Extensive studies have identified that many RNA-binding proteins, such as FUS, hnRNPA1, and TDP43, largely contribute to this conditional cellular compartmentation. These proteins commonly contain low complexity (LC) domains that can drive the full-length proteins to undergo liquid–liquid phase separation (LLPS) via weak multivalent interactions. In this work, we directly visualize temperature-sensitive amyloid fibrils in the liquid-like droplets of hnRNPA1 by transmission electron microscopy (TEM). Our work bridges the liquid phase and solid phase of hnRNPA1 and illuminates the functional role of reversible amyloids in the assembly of stress granules and the pathological risk as intermediates en route to irreversible fibrils.

As a control, we also determined the atomic structure of segment 234GGGYGGS240 by X-ray diffraction. This segment does not form fibrils or hydrogels and thus may not be an amyloid core. Indeed, the structure showed an unfolded conformation with no fibrillar packing.

>[2x]GGGYGGS> MKQFEIVIEPIQTEQYREFTINEYQGAVVVFTGHVREWTKGVKTEYLEYEAYIPMAEKKLAQIGDEINEKWPGTITSIVHRIGPLQISDIAVLIAV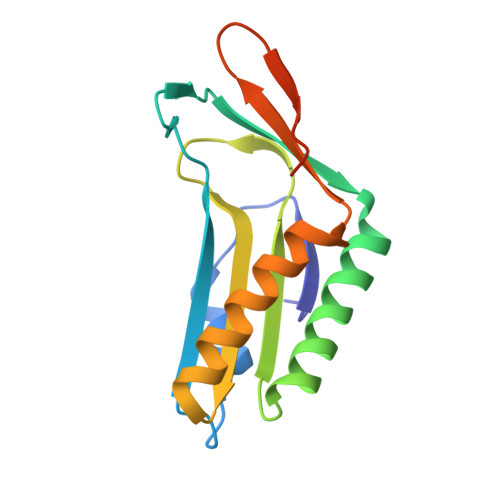SSPHRKDAYRANEYAIERIKEIVPIWKKEIWEDGSKWQGHQKGNYEEAKREE> DEREIARKVASELQKFSEWVKKL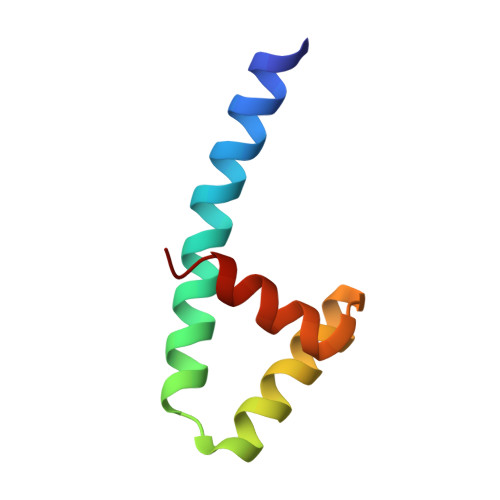KEVIKKASPEQQTKIAQWVAKLAGVRPEDVKKIIKAFND Here, we describe an AVV platform using phage T4. It contains a large 120 × 86 nm prolate icosahedral capsid (head) assembled with 930 molecules or 155 hexameric capsomers of the major capsid protein gp23* (* represents the cleaved mature form), 55 copies or 11 pentamers of gp24* at eleven of the twelve vertices, and 12 copies of the portal protein gp20 at the unique twelfth vertex. First, the architecture of T4 phage with a stable capsid and external surface exposing 1,025 nonessential molecules, and an internal volume that can accommodate up to ~171 Kbp DNA and ~1,000 molecules of internal proteins (IPs), provide ample cargo space to incorporate therapeutic biomolecules. Since the T4 capsid has a high density of negative charges, ~6,829 net negative charges per capsid, we hypothesized that cationic lipids would spontaneously assemble on T4 capsid via electrostatic interactions.

Next, we asked if the T4 capsid can be re-wired by CRISPR engineering such that it can be further programmed with a large number of foreign peptides, 930 or one per gp23* capsid protein subunit, on the capsid exterior. Peptides of various lengths consisting of aspartic acid (D) and glutamic acid (E) residues were inserted into the I domain loop by CRISPR engineering. Remarkably, the T4 capsid can tolerate up to 9 acidic residues (9DE) with no significant effect on plaque size or phage production. We then introduced 9DE-gp23, 10am, 13am, Hoc-del, and Soc-del mutations into the genome through CRISPR to generate 9DE-T4 phage (9DE-gp23.10-amber.13-amber.HocΔ.SocΔ T4) and heads for AVV assembly. A 3.9 Å high-resolution cryo-EM structure of 9DE-T4 head was generated, which showed decoration of the capsid with 9DE peptides between residues G201 and A202 of the I domain loops. The six 9DE peptides in each capsomer formed a negatively-charged acidic ring, generating an extraordinarily charged super-acidic capsid surface containing 8,370 additional negative charges per capsid (totally 15,199 net negative charges in 9DE-T4 compared to 6,829 in WT-T4). The 9DE-T4 heads bound strongly to anion-exchange columns requiring a much higher NaCl concentration to elute, and a slightly larger 9DE-gp23* band was also visualized by SDS-PAGE. A head-to-head comparison of WT-T4-AVVs and 9DE-T4-AVVs showed that packaging efficiency was not affected by acidification. Remarkably, however, head to head comparison of the AVVs assembled with the super-acidic heads exhibited ~5-fold greater transduction efficiency than the WT-AVVs, as measured by the delivered luciferase activity at MOIs of 103 and 104. Importantly, the enhanced transduction efficiency of the super-acidic AVVs was also recapitulated for delivery and expression of the full-length dystrophin payload.

>[93x]AEIGGDHGYNATNIAAGQTSGAVTQIGPAVMGMVRRAIPNLIAFDICGVQPMNSPTGQVFALRAVYGKDPVAAGAKEAFHPMYGPDAMFSGQGAAKKFPALAASTQTTVGDIYTHFFQETGTVYLQASVQVTIDAGDEDEDEDEDATDAAKLDAEIKKQMEAGALVEIAEGMATSIAELQEGFNGSTDNPWNEMGFRIDKQVIEAKSRQLKAAYSIELAQDLRAVHGMDADAELSGILATEIMLEINREVVDWINYSAQVGKSGMTLTPGSKAGVFDFQDPIDIRGARWAGESFKALLFQIDKEAVEIARQTGRGEGNFIIASRNVVNVLASVDTGISYAAQGLATGFSTDTTKSVFAGVLGGKYRVYIDQYAKQDYFTVGYKGPNEMDAGIYYAPYVALTPLRGSDPKNFQPVMGFKTRYGIGINPFAESAAQAPASRIQSGMPSILNSLGKNAYFRRVYVKGI;>[5x]STTTNSNSIGRPNLVALTRATTKLIYSDIVATQRTNQPVAAFYGIKYLNPDNEFTFKTGATYAGEAGYVDREQITELTEESKLTLNKGDLFKYNNIVYKVLEDTPFATIEESDLELALQIAIVLLKVRLFSDAASTSKFESSDSEIADARFQINKWQTAVKSRKLKTGITVELAQDLEANGFDAPNFLEDLLATEMADEINKDILQSLITVSKRYKVTGITDSGFIDLSYASAPEAGRSLYRMVCEMVSHIQKESTYTATFCVASARAAAILAASGWLKHKPEDDKYLSQNAYGFLANGLPLYCDTNSPLDYVIVGVVENIGEKEIVGSIFYAPYTEGLDLDDPEHVGAFKVVVDPESLQPSIGLLVRYALSANPYTVAKDEKEARIIDGGDMDKMAGRSDLSVLLGVKLPKIII>MVQPFAAQVASLADRYEESFDIGAAVEPHQLNGRQGKVLKHHYNSIVAENAMKPISLQPEEGVFTWDGADAIVEFARKNNMNLRFHTLVWHNQVPDWFFLDEEGNPMVEETNEAKRQANKELLLERLETHIKTVVERYKDDVTAWDVVNEVVDDGTPNERGLRESVWYQITGDEYIRVAFETARKYAGEDAKLFINDYNTEVTPKRDHLYNLVQDLLADGVPIDGVGHQAHIQIDWPTIDEIRTSMEMFAGLGLDNQVTELDVSLYGWPPRPAFPTYDAIPQERFQAQADRYNQLFELYEELDADLSSVTFWGIADN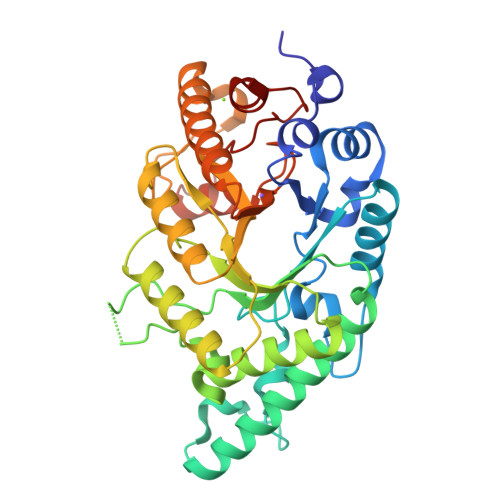HTWLDDRAREYNDGVGKDAPFVFDPNYRVKPAFWRIID[2x]> MAHHHHHHMQDEMYMARALKLAARGRFTTHPNPNVGCVIVKDGEIVGEGFHYRAGEPHAEVHALRMAGDKAKGATAYVTLEPCSHHGRTPPCCDALIAAGVARVVAAM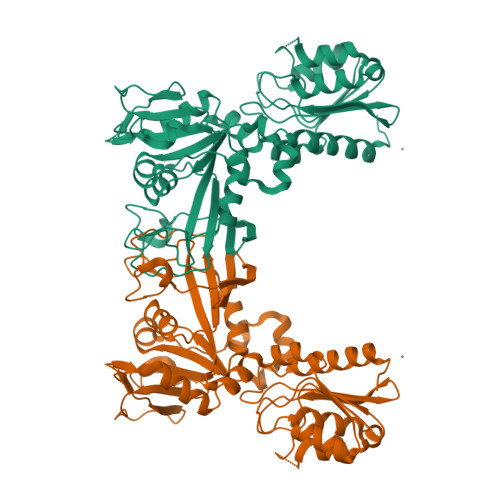QDPNPQVAGRGLYRLQQAGIDVSHGLMMNEAEALNKGFLKRMRTGFPWIQLKMGASLDGRTAMASGESQWITSPQARRDVQRLRAQSHAILTSSATVLADDPALTVRWQELSADTQALYPQENLRQPLRIVIDSQNRVTPEHRIIQQQGETLFARTHADERAWPDNVRTLLVPEHNGHLDLVLLMMQLGKQQVNSIWVEAGPTLAGALLQAGLVDELIVYIAPKLLGSDARGLCALPGLEKLSQAPHFKFNEIRQVGPDVCLHLTTA> MGSSHHHHHHENLYFQGHMENPANANPIRVGVIGCADIAWRRALPALEAEPLTEVTAIASRRWD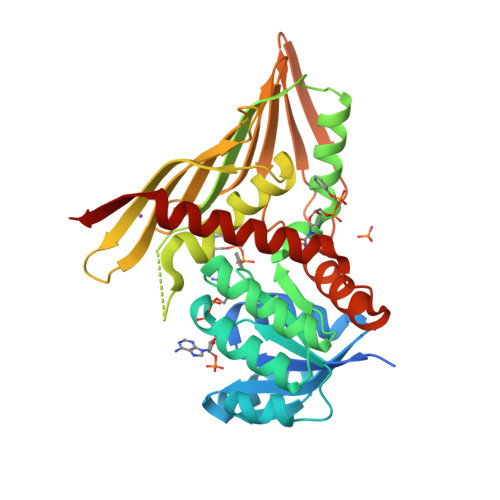RAKRFTERFGGEPVEGYPALLERDDVDAVYVPLPAVLHAEWIDRALRAGKHVLAEAPLTTDRPQAERLFAVARERGLLLMENFMFLHHPQHRQVADMLDEGVIGEIRSFAASFTIPPKPQGDIRYQADVGGGALLDIGVYPIRAAGLFLGADLEFVGAVLRHERDRDVVVGGNALLTTRQGVTAQLTFGMEHAYTNNYEFRGSTGRLWMNRVFTPPATYQPVVHIERQDHAEQFVLPAHDQFAKSIRAFAQAVLSGEHPREWSEDSLRQASLVDAVRTGARDIYFP> APAHADHQITKRTDAENMYNTIQFLSQAPRVAGSPEEL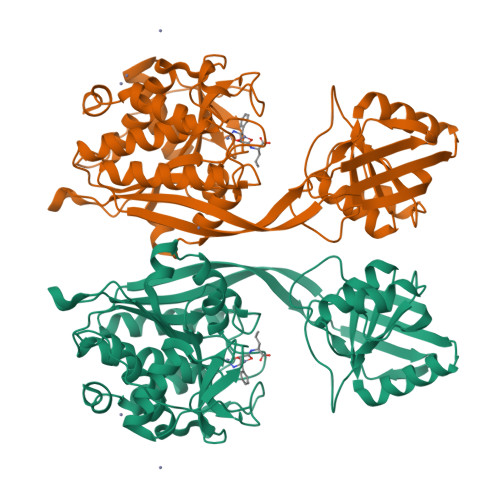KAVRYIEQQFKSYGYHVEVQPFQFEGYTAPSEVTLKIGTEKKEGEAFTYSPNSDVTAELVYVGLGTTADVAGKDLNGKIALIQRGNISFADKVRNAAKQGAKAVIIYNNTDGKLNGTLGGSDASFVAAVGITKQEGDALAANLRAGEKITATVKVAGAEVKTLTSHNVIATKKPDANKKNTNDIIIIGSHHDSVEKAPGANDDASGVAVTLELARVMSKLKTDTELRFITFGAEENGLIGSKKYAASLSEDEIKRTIGMFQLDMVGSKDAGDLIMYTIDGKKNRVTDLGAAASSRLSGVLPYGQEGRSDHESFHALGIPAALFIHAPVEPWYHTPNDTLDKISKEKLDNVADIVGSAVYQAARPGELVIEPIDYPRRNVELQN>GSPAEIASFSPRPSLADSKAVLNQAVADLSVAHSILHQVHWYMRGRGFMIWHPKMDEYMEEIDGYLDEMSERLITL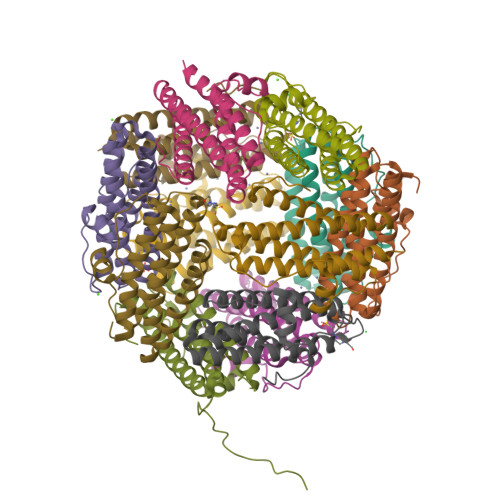GGAPFSTLKEFSENSQLKEVLGDYNVTIEEQLARVVEVFRYLAALFQKGFDVSDEEGDSVTNDIFNVAKASIEKHIWMLQAELGQAPKL[12x]>[4x]GSMELRVGNRYRLGRKIGSGSFGDIYLGTDIAAGEEVAIKLECVKTKHPQLHIESKIYKMMQGGVGIPTIRWCGAEGDYNVMVMELLGPSLEDLFNFCSRKFSLKTVLLLADQMISRIEYIHSKNFIHRDVKPDNFLMGLGKKGNLVYIIDFGLAKKYRDARTHQHIPYRENKNLTGTARYASINTHLGIEQSRRDDLESLGYVLMYFNLGSLPWQGLKAATKRQKYERISEKKMSTPIEVLCKGYP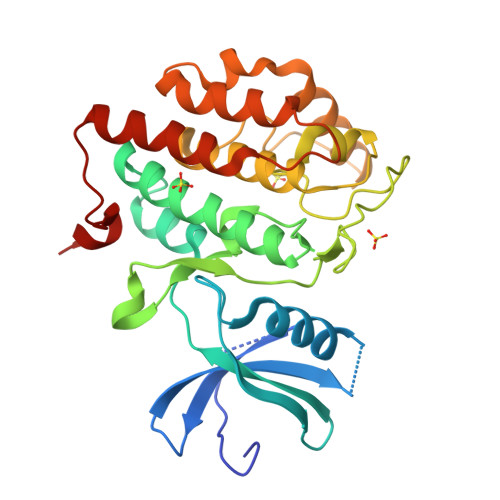SEFATYLNFCRSLRFDDKPDYSYLRQLFRNLFHRQGFSYDYVFDWNMLK2S,4R-4-METHYLGLUTAMATE | C6 H10 N O4 | 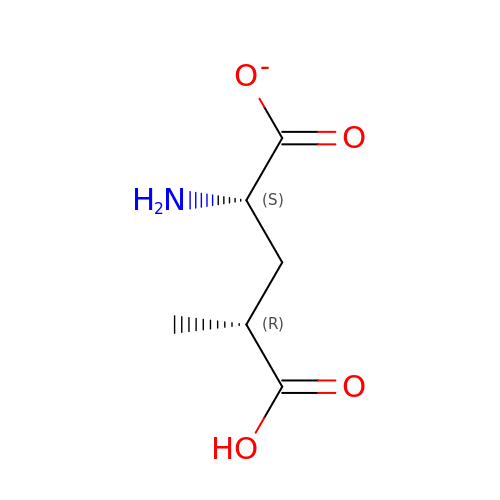KRKRAOXTGDJWNI-DMTCNVIQSA-M>GSHMTQDCSFQHSPISSDFAVKIRELSDYLLQDYPVTVASNLQDEELCGGLWRLVLAQRWMERLKTVAGSKMQGLLERVNTEIHFVTKCAFQPPPSCLRFVQTNISRLLQETSEQLVALKPWITRQNFSRCLELQCQP[4x];>[4x]ETGNQDLPVIKCVLINHKNNDSSVGKSSSYPMVSESPEDLGCALRPQSSGTVYEAAAVEVDVSASITLQVLVDAPGNISCLWVFKHSSLNCQPHFDLQNRGVVSMVILKMTETQAGEYLLFIQSEATNYTILFTVSIRNTLLYTLRRPYFRKMENQDALVCISESVPEPIVEWVLCDSQGESCKEESPAVVKKEEKVLHELFGTDIRCCARNELGRECTRLFTIDLNQTPQTTLPQLFLKVGEPLWIRCKAVHVNHGFGLTWELENKALEEGNYFEMSTYSTNRTMIRILFAFVSSVARNDTGYYTCSSSKHPSQSALVTIVEKGFINATNSSEDYEIDQYEEFCFSVRFKAYPQIRCTWTFSRKSFPCEQKGLDNGYSISKFCNHKHQPGEYIFHAENDDAQFTKMFTLNIRRKPQVLAEASASQASCFSDGYPLPSWTWKKCSDKSPNCTEEITEGVWNRKANRKVFGQWVSSSTLNMSEAIKGFLVKCCAYNSLGT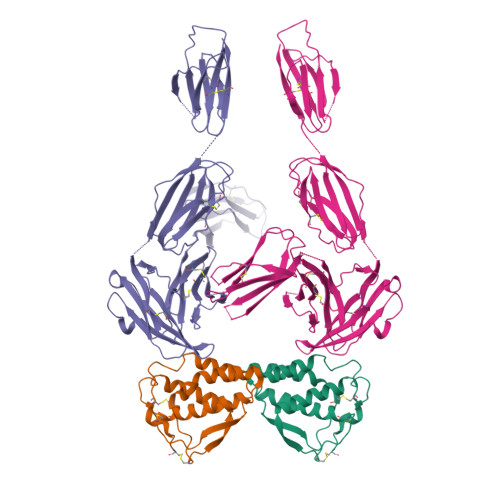SCETILLNSPGPFPFIQDGGTKHHHHHH> MINQEKRPFRIRDKYIDRDSEYLLQENEPDATLDQQLLEDLQKKKTDLRYIEMQRFREKLPSYGMQKELVNMIDNHQVTVISGETGCGKTTQVTQFILDNYIERGKGSACRIVCTQPRRISAISVAERVAAERAESCGNGNSTGYQIRLQSRLPRKQGSILYCTTGIILQWLQSDPHLSSVSHIVLDEIHERNLQSDVLMTVVKDLLSYRPDLKVVLMSATLNAEKFSEYFGNCPMIHIPGFTFPVVEYLLEDIIEKIRYVPEQKEHRSQFKKGFMQGHVNRQEKYYYEAIYKERWPGYLRELRQRYSASTVDVVEMMDDEKVDLNLIAALIRYIVLEEEDGAILVFLPGWDNISTLHDLLMSQVMFKSDKFIIIPLHSLMPTVNQTQVFKRTPPGVRKIVIATNIAETSITIDDVVYVIDGGKIKETHFDTQNNISTMSAEWVSKANAKQRKGRAGRVQPGHCYHLYNSLRASLLDDYQLPEILRTPLEELCLQIKILRLGGIAHFLSRLMDPPSNEAVLLSIKHLMELNALDKQEELTPLGVHLARLPVEPHIGKMILFGALFCCLDPVLTIAASLSFKDPFVIPLGKEKVADARRKELAKDTKSDHLTVVNAFKGWEKAKQRGFRYEKDYCWEYFLSSNTLQMLHNMKGQFAEHLLGAGFVSSRNPQDPESNINSDNEKIIKAVICAGLYPKVAKIRLNLGKKRKMVKVYTKTDGVVAIHPKSVNVEQTEFNYNWLIYHLKMRTSSIYLYDCTEVSPYCLLFFGGDISIQKDNDQETIAVDEWIIFQSPARIAHLVKELRKELDILLQEKIESPHPVDWKDTKSRDC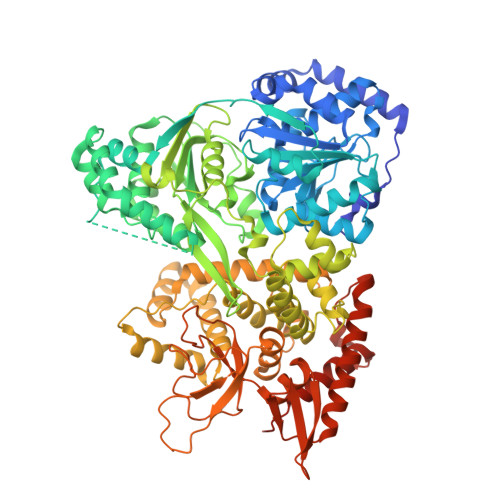AVLSAIIDLIKTQEKATPRNLPPRFQDGYYSPHHHHHHHH>[3x]MFSKLAHLQRFAVLSRGVHSSVASATSVATKKTVQGPPTSDDI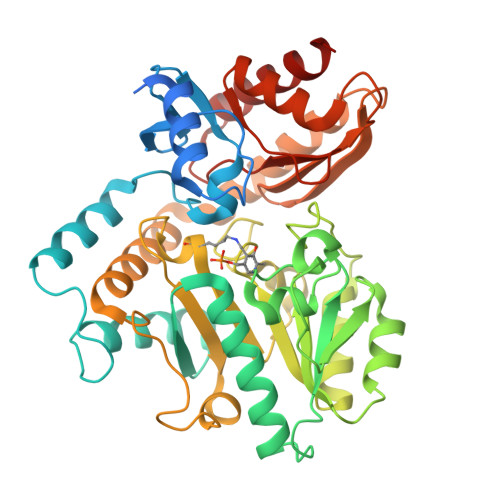FEREYKYGAHNYHPLPVALERGKGIYLWDVEGRKYFDFLSSYSAVNQGHCHPKIVNALKSQVDKLTLTSRAFYNNVLGEYEEYITKLFNYHKVLPMNTGVEAGETACKLARKWGYTVKGIQKYKAKIVFAAGNFWGRTLSAISSSTDPTSYDGFGPFMPGFDIIPYNDLPALERALQDPNVAAFMVEPIQGEAGVVVPDPGYLMGVRELCTRHQVLFIADEIQTGLARTGRWLAVDYENVRPDIVLLGKALSGGLYPVSAVLCDDDIMLTIKPGEHGSTYGGNPLGCRVAIAALEVLEEENLAENADKLGIILRNELMKLPSDVVTAVRGKGLLNAIVIKETKDWDAWKVCLRLRDNGLLAKPTHGDIIRFAPPLVIKEDELRESIEIINKTILSF>GHMPSSGKRRAPRRVYQIPQRRRLQGKDPRWATMADLKMQAVKEICYEVALADFRHGRAEIEALAALKMRELCRTYGKPDGPGDAWRAVARDVWDTVGE[2x];>GHMEKLHEANNELQKKRAIIEDLEPRFNNSSLKIEELQEALRKKEEEMKQMEERYKKYLEKAKSVIRTLDPKQNQ[2x]

Hook microtubule tethering protein 3 (Hook3), a cargo adaptor protein that serves as a crucial scaffold protein linking cargo to microtubule motors, plays a pivotal role in regulating bidirectional early endosome trafficking, managing directional movement, and maintaining Golgi morphology. Among these domains, the Hook domain together with the first and second coiled coils serve as the dynein-binding region, whereas the third coiled coil-containing the carboxyl-terminal region interacts with several proteins, including fused toes homolog (FTS), FTS−Hook−FHIP1B (FHF) complex subunit Hook interacting protein 1B (FHIP1B), and kinesin family member 1 C (KIF1C). KIF1C, a kinesin-3 family member with plus-end-directed motility, mediates the anterograde (plus-end-directed) transport of vesicles containing several components, such as α5β1 integrin, 14-3-3, and protein tyrosine phosphatase non-receptor type 21 (PTPN21). A previous study showed that KIF1C exists as an autoinhibited homodimer, and becomes activated by interacting with the carboxyl-terminal region of Hook3 or the FERM domain of PTPN21.

We verified the direct intermolecular interaction between Hook3 and KIF1C, and revealed their binding modules, which subsequently led to determination of the crystal structure of Hook3(553–624) bound to KIF1C(714–809) in a 2:2 heterotetrameric form. In this complex, residues 553–618 of Hook3, which constitute the parallel coiled coil, consist of two distinct types of heptad repeats (Fig. EV2). As shown in Fig. EV2B, the coiled-coil conformation of Hook3 is maintained by an elaborate network of hydrophobic interactions. This homodimeric Hook3 coiled-coil acts as a scaffold for complex formation with two KIF1C(714–809) molecules, in which residues 742–786 and 793–807 are visible in our complex crystal structure. KIF1C(714–809) forms an antiparallel three-helical bundle consisting of α1 (residues 744–762), α2 (residues 768–785), and α3 (residues 795–807). The protein folding of KIF1C(714–809) is sustained by intensive intramolecular hydrophobic interactions between the residues constituting the three α-helices, which include Lys748, Val752, Ile755, and Val759 from α1; Phe764 from the α1–α2 loop; Ile771, Ala775, Ala776, and Met779 from α2; Trp796, Val799, Ala800, Val803, Trp804, and Val807 from α3 (Fig. EV3A). Our crystal structure revealed several key hydrophobic residues from the α1 helix and the α1–α2 loop of KIF1C that directly contribute to the complex formation, in which each single KIF1C protomer recognizes both molecules of homodimeric Hook3. Specifically, the main Hook3-binding interface of KIF1C is constituted by Lys753, Tyr757, Ala760, and Leu761 from α1; Asp763 and Phe764 from the α1–α2 loop, which are associated with Tyr607, Lys610, Ala611, Val614, and Leu618 of one Hook3 molecule and Lys612, Ile615, Arg616, and Pro620 of another Hook3 protomer that coordinately form a large extended hydrophobic surface on the Hook3 homodimer (Figs. 2C and EV3B).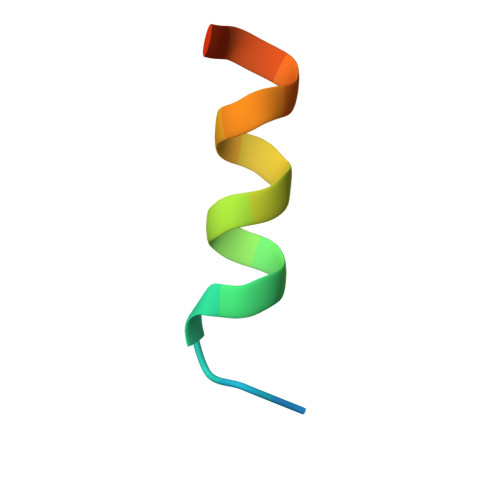> SREKPYKEVTEDLLHLNSLF> 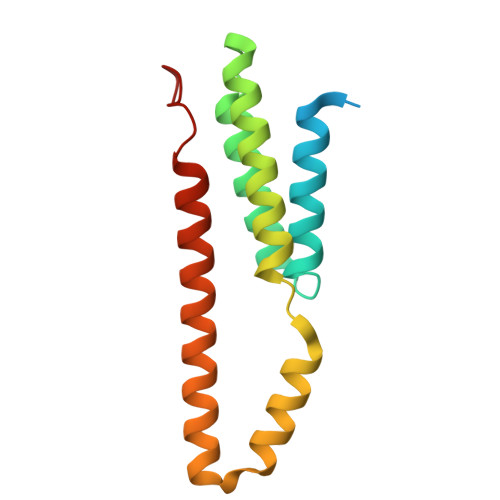MNCSSTLACHAVVSAPSTASLITSCWTPQQHCYRQLMKSLRAAYFHDRSKLFWSRHRVLVEFYKYSEEANEEAVKQLVAIGLEVAAFIDHHMRTDVERIVKHNETMMALPVAQAKKFRSDYLLAEKQHDSWCKQKIKNIMKRRPPPPYPFF> MHYQPKQDLLNDRIILVTGASDGIGREAAMTYARYGATVILLGRNEEKLRQVASHINEETGRQPQWFILDLLTCTSENCQQLAQRIAVNYPRLDGVLHNAGLLGD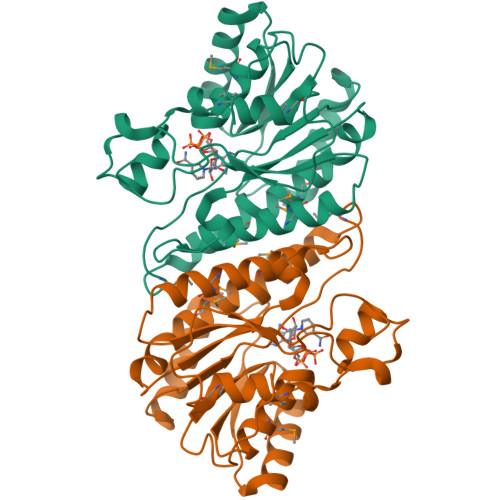VCPMSEQNPQVWQDVMQVNVNATFMLTQALLPLLLKSDAGSLVFTSSSVGRQGRANWGAYAASKFATEGMMQVLADEYQQRLRVNCINPGGTRTAMRASAFPTEDPQKLKTPADIMPLYLWLMGDDSRRKTGMTFDAQPGRKPGISQ> MAFHEVRFPANLSFGSVGGPERRTEIVTLSSGHEERNSPWAHSRRHYDAGVGLRSLDDVERLIAFFE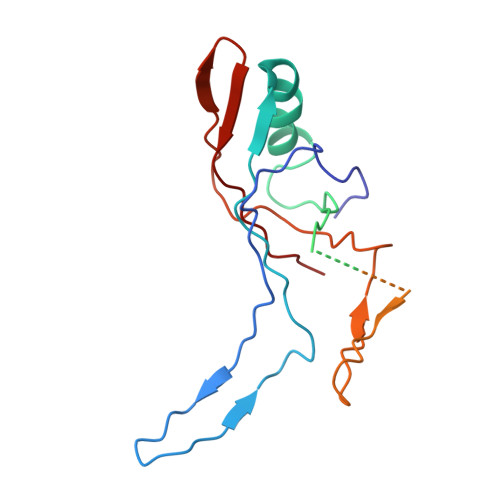ARGGQLHGFRWKDWADFKSCPASRAVAHEDQLIGMGDGVTTAFQLVKTYVSGGQSYLRPIVKPVEGTVKLGIAGDHQAEAVNFAVDHATGIVSFNEPPPQGARVTAGFEFDVPVRFDTDRIAVSVQSFQAGDLPQVPVVEVRI> MNILSKISSFIGKTFSLWAALFAAAAFFAPDTFKWAGPYIPWLLGIIMFGMGLTLKPSDFDILFKHPKVVIIGVIAQFAIMPATAWLLSKLLNLPAEIAVGVILVGCCPGGTASNVMTYLARGNVALSVAVTSVSTLISPLLTPAIFLMLAGEMLEIQAAGMLMSIVKMVLLPIVLGLIVHKVLGSKTEKLTDALPLVSVAAIVLIIGAVVGASKGKIMESGLLIFAVVVLHNGIG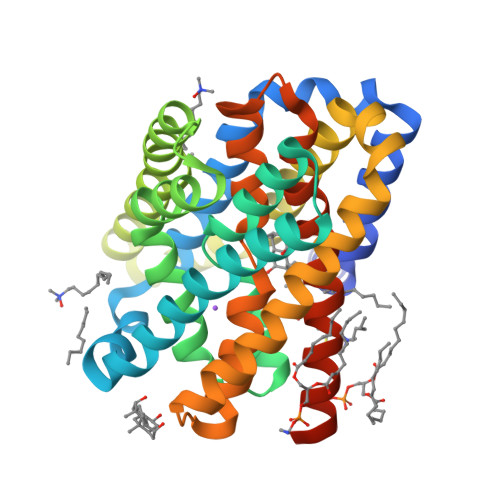YLLGFFAAKWTGLPYDAQKTLTIEVGMQNSGLAAALAAAHFAAAPVVAVPGALFSVWHNISGSLLATYWAAKAGKHKKPGSENLYFQ>[5x]MQLQELHMLVVLAEELNMRKAAERLFVSQPALSQRLQTIEKAWGTKIFLRSQKGLTVTPAGEKIIQFANDVTDRQERIRENIDELEGEIHGTLKLAVASIIGQHWLPKVLKTYVERYPNAKVSLITGWSSEMLKSLYEDQVHIGIIRGNPEWKGRKDYLMTDHLYLVDTEISCIDDIAHTDRPFIQFKSDSTYFQEIQHWWHQKFKTSPKQTILVDQIETCKQMALH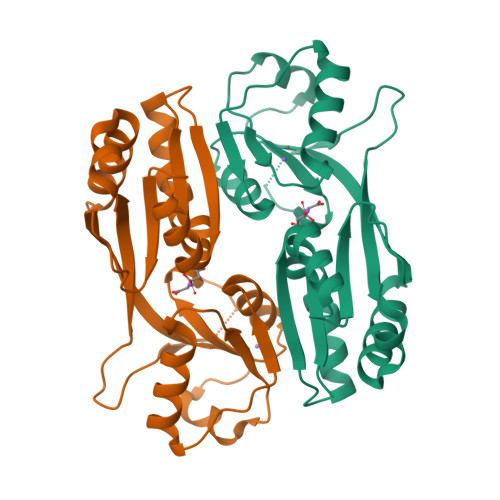GIGYAILPSVTLEEEDKVNKMPLLDTKDHPIGRDTWLLGYEPAFELKQVQAFVSVIKDMLKQERPF(2~{R},3~{S},4~{S},5~{R},6~{S})-2-(hydroxymethyl)-6-[(2~{R},3~{R},4~{S},5~{R},6~{S})-2-(hydroxymethyl)-6-[(2~{R},3~{R},4~{S},5~{R},6~{R})-2-(hydroxymethyl)-3,5-bis(oxidanyl)-6-[4-(3-quinolin-1-ium-1-ylpropyl)-1,2,3-triazol-1-yl]oxan-4-yl]oxy-3,5-bis(oxidanyl)oxan-4-yl]oxy-oxane-3,4,5-triol 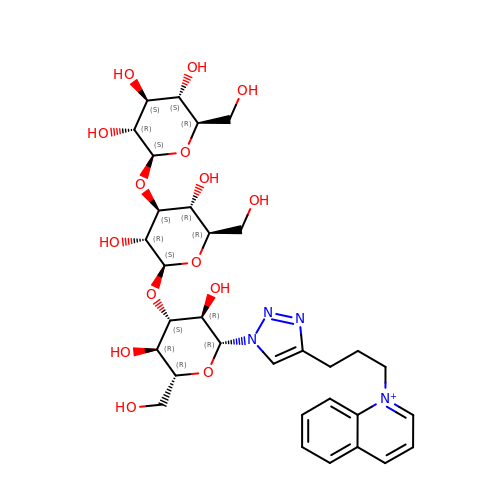| C32 H45 N4 O15 | ZDLMHTZQWQBSDO-DGUZUYFASA-N>MAEESRGQRGSGYGLGLSTRTQVTGYQFLARRTAMALTRWRVRMEIEPGRRQTLAVVASVSAALVICLGALLWSFISPSGQLNESPIIADRDSGALYVRVGDRLYPALNLASARLITGRPDNPHLVRSSQIATMPRGPLVGIPGAPSSFSPKSPPASSWLVCDTVATSSSIGSLQGVTVTVIDGTPDLTGHRQILSGSDAVVLRYGGDAWVIREGRRSRIEPTNRAVLLPLGLTPEQVSQARPMSRALFDALPVGPELLVPEVPNAGGPATFPGAPGPIGTVIVTPQISGPQQYSLVLGDGVQTLPPLVAQILQNAGSAGNTKPLTVEPSTLAKMPVVNRLDLSAYPDNPLEVVDIREHPSTCWWWERTAGENRARVRVVSGPTIPVAATEMNKVVSLVKADTSGRQADQVYFGPDHANFVAVTGNNPGAQTSESLWWVTDAGARFGVEDSKEARDALGLTLTPSLAPWVALRLLPQGPTLSRADALVEHDTLPMDMTPAELVVPK[6x];>[6x]MKRGFARPTPEKPPVIKPENIVLSTPLSIPPPEGKPWWLIVVGVVVVGLLGGMVAMVFASGSHVFGGIGSIFPLFMMVGIMMMMFRGMGGGQQQMSRPKLDAMRAQFMLMLDMLRETAQESADSMDANYRWFHPAPNTLAAAVGSPRMWERKPDGKDLNFGVVRVGVGMTRPEVTWGEPQNMPTDIELEPVTGKALQEFGRYQSVVYNLPKMVSLLVEPWYALVGEREQVLGLMRAIICQLAFSHGPDHVQMIVVSSDLDQWDWVKWLPHFGDSRRHDAAGNARMVYTSVREFAAEQAELFAGRGSFTPRHASSSAQTPTPHTVIIADVDDPQWEYVISAEGVDGVTFFDLTGSSMWTDIPERKLQFDKTGVIEALPRDRDTWMVIDDKAWFFALTDQVSIAEAEEFAQKLAQWRLAEAYEEIGQRVAHIGARDILSYYGIDDPGNIDFDSLWASRTDTMGRSRLRAPFGNRSDNGELLFLDMKSLDEGGDGPHGVMSGTTGSGKSTLVRTVIESLMLSHPPEELQFVLADLKGGSAVKPFAGVPHVSRIITDLEEDQALMERFLDALWGEIARRKAICDSAGVDDAKEYNSVRARMRARGQDMAPLPMLVVVIDEFYEWFRIMPTAVDVLDSIGRQGRAYWIHLMMASQTIESRAEKLMENMGYRLVLKARTAGAAQAAGVPNAVNLPAQAGLGYFRKSLEDIIRFQAEFLWRDYFQPGVSIDGEEAPALVHSIDYIRPQLFTNSFTPLEVSVGGPDIEPVVAQPNGEVLESDDIEGGEDEDEEGVRTPKVGTVIIDQLRKIKFEPYRLWQPPLTQPVAIDDLVNRFLGRPWHKEYGSACNLVFPIGIIDRPYKHDQPPWTVDTSGPGANVLILGAGGSGKTTALQTLICSAALTHTPQQVQFYCLAYSSTALTTVSRIPHVGEVAGPTDPYGVRRTVAELLALVRERKRSFLECGIASMEMFRRRKFGGEAGPVPDDGFGDVYLVIDNYRALAEENEVLIEQVNVIINQGPSFGVHVVVTADRESELRPPVRSGFGSRIELRLAAVEDAKLVRSRFAKDVPVKPGRGMVAVNYVRLDSDPQAGLHTLVARPALGSTPDNVFECDSVVAAVSRLTSAQAPPVRRLPARFGVEQVRELASRDTRQGVGAGGIAWAISELDLAPVYLNFAENSHLMVTGRRECGRTTTLATIMSEIGRLYAPGASSAPPPAPGRPSAQVWLVDPRRQLLTALGSDYVERFAYNLDGVVAMMGELAAALAGREPPPGLSAEELLSRSWWSGPEIFLIVDDIQQLPPGFDSPLHKAVPFVNRAADVGLHVIVTRTFGGWSSAGSDPMLRALHQANAPLLVMDADPDEGFIRGKMKGGPLPRGRGLLMAEDTGVFVQVAATEVRR;>[12x]MTAVADAPQADIEGVASPQAVVVGVMAGEGVQIGVLLDANAPVSVMTDPLLKVVNSRLRELGEAPLEATGRGRWALCLVDGAPLRATQSLTEQDVYDGDRLWIRFIADTERRSQVIEHISTAVASDLSKRFARIDPIVAVQVGASMVATGVVLATGVLGWWRWHHNTWLTTIYTAVIGVLVLAVAMLLLMRAKTDADRRVADIMLMSAIMPVTVAAAAAPPGPVGSPQAVLGFGVLTVAAALALRFTGRRLGIYTTIVIIGALTMLAALARMVAATSAVTLLSSLLLICVVAYHAAPALSRRLAGIRLPVFPSATSRWVFEARPDLPTTVVVSGGSAPVLEGPSSVRDVLLQAERARSFLSGLLTGLGVMVVVCMTSLCDPHTGQRWLPLILAGFTSGFLLLRGRSYVDRWQSITLAGTAVIIAAAVCVRYALELSSPLAVSIVAAILVLLPAAGMAAAAHVPHTIYSPLFRKFVEWIEYLCLMPIFPLALWLMNVYAAIRYR;>MQRFGTGSSRSWCGRAGTATIAAVLLASGALTGLPPAYAISPPTIDPGALPPDGPPGPLAPMKQNAYCTEVGVLPGTDFQLQPKYMEMLNLNEAWQFGRGDGVKVAVIDTGVTPHPRLPRLIPGGDYVMAGGDGLSDCDAHGTLVASMIAAVPANGAVPLPSVPRRPVTIPTTETPPPPQTVTLSPVPPQTVTVIPAPPPEEGVPPGAPVPGPEPPPAPGPQPPAVDRGGGTVTVPSYSGGRKIAPIDNPRNPHPSAPSPALGPPPDAFSGIAPGVEIISIRQSSQAFGLKDPYTGDEDPQTAQKIDNVETMARAIVHAANMGASVINISDVMCMSARNVIDQRALGAAVHYAAVDKDAVIVAAAGDGSKKDCKQNPIFDPLQPDDPRAWNAVTTVVTPSWFHDYVLTVGAVDANGQPLSKMSIAGPWVSISAPGTDVVGLSPRDDGLINAIDGPDNSLLVPAGTSFSAAIVSGVAALVRAKF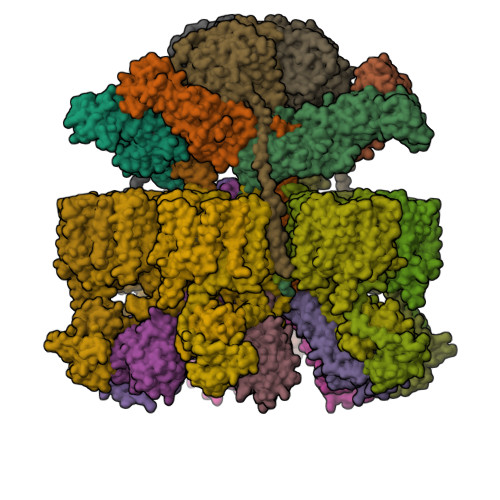PELSAYQIINRLIHTARPPARGVDNQVGYGVVDPVAALTWDVPKGPAEPPKQLSAPLVVPQPPAPRDMVPIWVAAGGLAGALLIGGAVFGTATLMRRSRKQQ[3x]>[4x]MNTPEHMTAVVQRYVAALNAGDLDGIVALFADD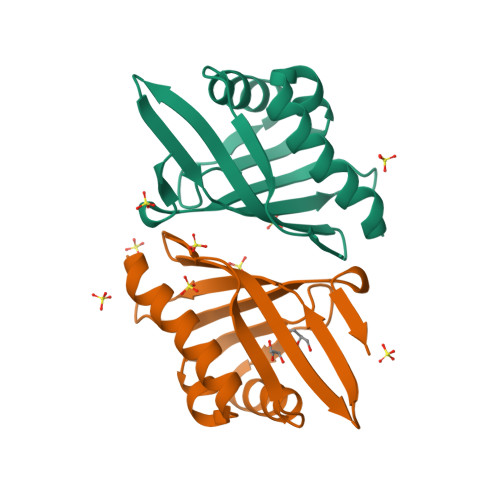ATVEEPVGSEPRSGTAAIREFYANSLKLPLAVELTQEVRAVANEAAFAFTVSFEYQGRKTVVAPINHFRFNGAGKVVSMRALFGEKNIHAGA1~{H}-indole-5-carboxamide | C9 H8 N2 O | 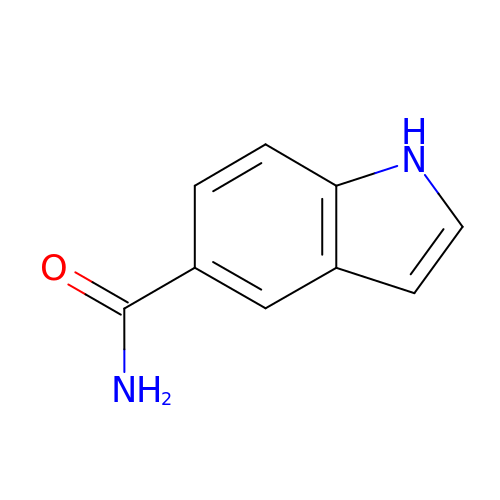GQMYQEAXTITUAE-UHFFFAOYSA-N> SNPLIRKAMGMDTEGGGKDEKMSGLRAEPTLKHFDENIISLIESEIMSVNNEIGWADVAGLEGAKKALREIVVLPFKRPDVFTGIRAPPKGVLLFGPPGTGKTMIGRCVASQCKATFFNISASSLTSKWVGEGEKLVRALFSVARLKLPSVIFIDEIDSLLSSRSESEHESSRRIKTEFLVQLDGVNTAPDERLLVLGATNRPQELDEAARRRFQKRLYIALPEPESRTQIVQNLLVGT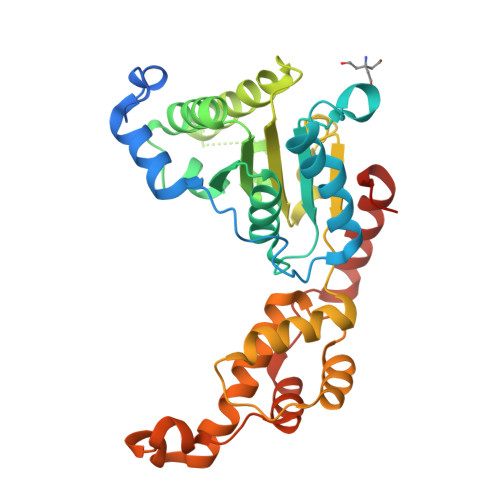RHDITNHNLERIRELTDGYSGADMRQLCTEAAMGPIRDIGDDIETIDKDDIRAVTVMDFAEAARVVRPTVDDSQLDAYAAWDKKFGCLPPPSISR> YHYEHETHAPLSPRIRKVGDIEF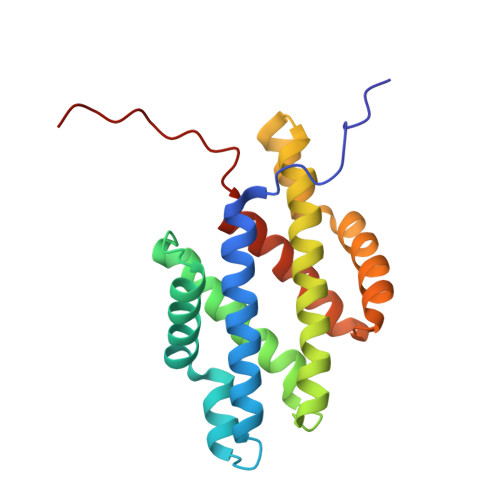HACSDYIYLLMTLSKDPEKFNYALKDRVSIRRYVRKNQNRYNYFLIEERVQDNIVNRISDRLISYCTDKEVTEDYIKKIDDYLWVEQRVIEEVSINVDHAREVKEKKRIMNDKKLIRMLFDTYEYVKDVKFTDDQYKDAAARISQFLIDVVDSYIIKPIPALP> MTVLHWATISPFLLAILIPFLYKYARRIHTGWFVLALPLVLFIYFIRYLSVTSTGGVVEHTIPWVPSLGINFTVFVDGLSLLFALLITGIGTLVILYSIFYLSKKTESLNNFYVYLLMFMGAMLGVVLSDNLIVLYVFWELTSLASSLLISYWFHREKSTYGAQKSMLITVFGGFAMLGGFSLLYVMTGTFSIRGIIENVDLVTSSELFLPAMILVLLGAFTKSAQFPFHIWLPDAMEAPTPVSAYLHSATMVKAGIYLVARLTPVFAGSAEWFWLLTGFGVVTLLWGSTSAVRQKDLKGILAFSTVSQLGLIMTLLGLGSAAIYFGDSVDPAFYSFAIMAAIFHLINHATFKGSLFMTAGIIDHETGTRDIRKLGGLMAIMPVTFTVSLIGLASMAGLPPFNGFLSKEMFFTALLRATEMNTFNMETFGIIIVVLAWIASVFTFLYCLIMFFKTFTGKFKPENYDVKVHEAPIGMLISPVILGSLVIVFGFFPNILAYTIIEPAMQAILPTLLADGEVFYVNIYMWHGFNAELFMTMGVVAAGIILFLMMKNWAKTAFYMKERDPLNWFYDNSLSGVITGSQAVTRIQMTGLLRDYFAYMTTFMILLLGYTMFRYDAFTIDTTNVTGIAPYIWVITLVFIAATLSIPFINKRITAVVVVGVIGFLLALLFVVFRAPDLALTQLLVETVTVLLLMLAFYHLPELRKEEFKPRFNIVNLIISIGVGFLVTAIALSSLALGNEAGIEPISQFFVENSKELAGGYNMVNVILVDFRGLDTLLEVLVLGIAALGVIALIKLRMTGREDV;> MKNLKSNDVLLHSVTRVVTFIILAFSVYLFFAGHNNPGGGFIGGLMTASALLLMYLGFDMKSIKKAIPFDFTKMIAFGLLLAIITGFGGLLVGDPYLTQYFEYYQIPILGETELTTALPFDLGIYLVVVGIALTIILTIAEDDM;> MEILMSITVGVLFMVGTYLILTKSLLRVVVGLILLSHGAHLLLLTMAGLQRGAPPLLHLEATTYSDPLPQALILTAIVISFGVTSFLLVLAYRTYKEHKTDDLDQLRGSADE;> MNNLVILPILIPFIVGTILILFAKNHSLQRVISGFTVIGMLLVAIYLAMDVYQNGISVLELGNWQAPFGIVLVADMFATMMVILASIVGVVCLFFAFQTISSEREKYYFYPFYFFLLAGVNGAFLTGDLFNLFVFFEVMLIASYILIVLGGTKYQLRESLKYVMINVFASILFIVGVAYIYSVTGTLNMADLAVKVGQLEQTGVLNVIAVIFLVVFAMKGGLFPLYFWLPRSYYGPPAAIAALFGGLLTKVGIYAIMRTFTLIFTHDPDFTHMLILILAGLTMFFGVLGAVSQFDFKRILSYHIISQVGYMVMGLGIYTQLAIAGAIYYIAHHIIVKAALFLFAGATQRITGTTDLKKMGGLLKTHPWLAWMFFISAISLAGIPPLSGFFSKFALILAAFLNENYIIAAVALAVGLLTLFSMMKIFIYAFWGEQKHTEQQANFKVGKLLLPIVPLVALTIILGFAAEPIFQYSLQVADQILDPTIYIESVLKE;>[2x]MAFQILLNLVIAVIWVNFQNSYTAVDFLIGYVVGIFILFVLRRFLRFDFYMRRVWAIIKLIVLFFKELILANIDVIKIVLSPKMNIQPGIVAVPTKLKTDWELSLLASLISLTPGTLSMDFSDDNKYIYIHAIDVPNKEKMIRDIHDTFERAILEVTN;> MFQSILMIVLVVMSISLFVCFIRTLIGPTMSDRIVALDTFGINLIGFIGVIMMLQETLAYSEVVLVISILAFIGSIALSKFIERGVVFDRG;> MTAVEIIISIFVLIGGFLSLLGSIGIIRFPDVYGRLHAATKSATLGVISIMLATFLFFFLVHGEFVGKLLLTILFVFLTAPVAGMMMGRSAYRVGVPLWEKSTQDDLKKMYEKKMKGSNHHHHHHDYKDDDDK

Multiple resistance and pH adaptation (Mrp) cation/proton antiporters are essential for growth of a variety of halophilic and alkaliphilic bacteria under stress conditions. The CPA3 family comprises the larger Mrp (multiple resistance and pH adaptation) type antiporters which have received much attention because of their evolutionary relationship to redox-driven ion pumps of the complex I superfamily. Group I Mrp antiporters consist of seven proteins (MrpA-MrpG). The stoichiometry of the Mrp type antiporters is unknown but is predicted to be electrogenic with the number of transferred protons exceeding the number of transferred sodium ions.

In this work, we determine the cryoEM structure of the Mrp antiporter from Bacillus pseudofirmus at 2.2 Å resolution. The final 3D reconstruction of the protomer yielded a 2.2-Å map, allowing us to build a model including 1957 amino acid residues, three phospholipids, and 360 water molecules. Most of the 360 modelled water molecules are located on the hydrophilic protein surfaces exposed to the cytoplasm or periplasm as expected, but about 70 water molecules are found in the interior of the trans-membrane region. During model building, we noticed clear alternative side chain positions A and B (called alternate locations or altloc in the pdb) for several residues and conformational variations for short sequence stretches. Furthermore, we observed a pronounced structural rearrangement in a highly conserved sequence stretch close to the N-terminal end of TMH8 (positions 246 to 252), resulting in alternative positions of several residues, including strictly conserved His248MrpA. In MrpA, His248MrpA is located at the junction of three hydrated pathways. In the C-terminal domain of MrpA, we modelled Glu687MrpA in TMH19 with two alternative positions of its side chain. With a probe radius of 1.2 Å we identified a putative sodium-exit tunnel originating above the strictly conserved Phe41MrpB that is separated from Glu687MrpA by the hydrophobic Ile77MrpC and Val686MrpA. Strikingly, the tunnel is blocked by one of the two alternative conformations of Phe41MrpB, suggesting a gating function for this residue.> ANTSSAYNSVYDFLRYHDRGDGLTVNGKTSYSIDQAAAQITRENVSWNGTNVFGKSANLTFKFLQSVSSIPSGDTGFVKFNAEQIEQAKLSLQSWSDVANLTFTEVTGNKSANITFGNYTRDASGNLDYGTQAYAYYPGNYQGAGSSWYNYNQSNIRNPGSEEYGRQTFTHEIGHALGLAHPGEYNAGEGDPSYNDAVYAEDSYQFSIASYWGENETGADYNGHYGGAPMIDDIAAIQRLYGANMTTRTGDSVYGFNSNTDRDFYTATDSSKALIFSVWDAGGTDTFDFSGYSNNQRINLNEGSFSDVGGLKGNVSIAHGVTIENAIGGSGNDILVGNSADNILQGGAGNDVLYGGAGADTLYGGAGRDTFVYGSGQDSTVAAYDWIADFQKGIDKIDLSAFRNEGQLSFVQDQFTGKGQEVMLQWDAANSIT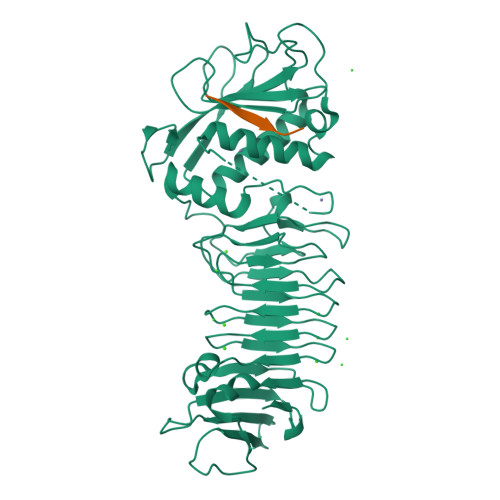NLWLHEAGHSSVDFLVRIVGQAAQSDIIV;> AKASQAA>[2x]HMTEEEVRKIMEKLKKAFKQGNPEQIVSLLSPDVKVDVGNQSFSG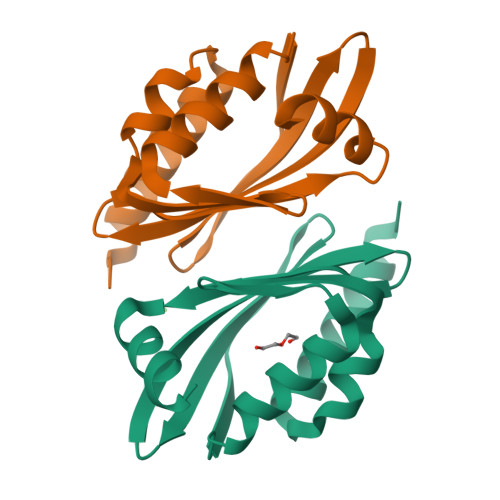SEEAEKMWRKLMKFVDRVEVRDVRVFENAVMIAVEFEVNGQRYKMIFTFYVENGKVSMVSIYISPTMKKLMKQILNYG>GSKNAPSTAGLGYGSWEIDPKDLTFLKELGTGQFGVVKYGKWRGQYDVAIKMIKEGSMSEDEFIEEAKVMMNLSHEKLVQLYGVCTKQRPIFIITEYMANGCLLNYLREMRHRFQTQQLLEMCKDVCEAMEYLESKQFLHRDLAARNCLVNDQGVVKVSDFGLSRYVLDDEYTSSVGSKFPVRWSPPEVLMYSKFSSKSDIWAFGVLMWEIYSLG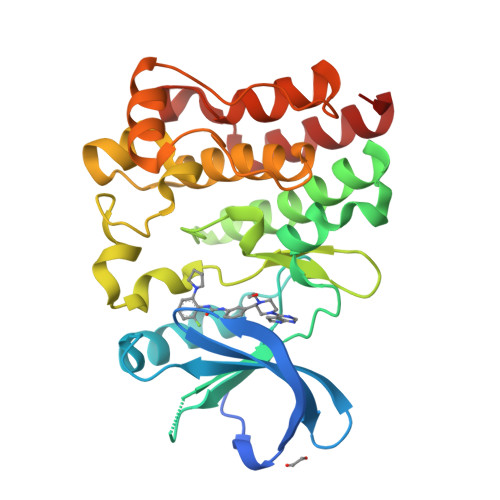KMPYERFTNSETAEHIAQGLRLYRPHLASEKVYTIMYSCWHEKADERPTFKILLSNILDVMDEES[2x]> GSHMDELAPPKPPLPEGEVPPPRPPPPEEKDEEFPEQKAGEVINQPMMMAARQLHDEARKWSSKPGIPAAEVGIGVVAEADAADAAGFPVPPDMEDDYEPELLLMPSNQPVNQPILAAAQSLHREATK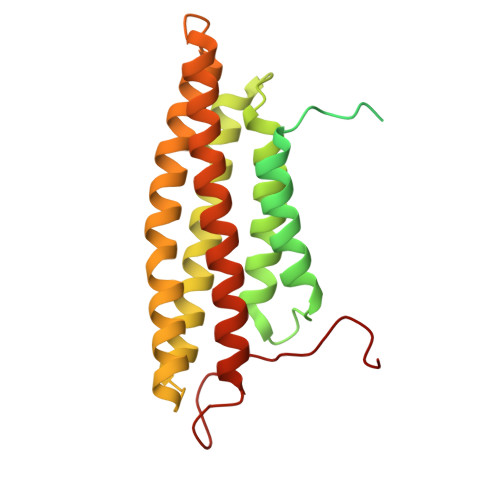WSSKGNDIIAAAKRMALLMAEMSRLVRGGSGTKRALIQCAKDIAKASDEVTRLAKEVAKQCTDKRIRTNLLQVCERIPTISTQLKILSTVKATMLGRTNISDEESEQATEMLVHNAQNLMQSVKETVREAEAASIKIRTDAGFTLRWVRKTPWYQ> MMFGKKKNNGGSSTARYSAGNKYNTLSNNYALSAQQLLNASKIDDIDSMMGFERYVPPQYNGRFDAKDIDQIPGRVGWLTNMHATLVSQETLSSGSNGGGNSNDGERVTTNQGISGVDFYFLDEEGGSFKSTVVYDPYFFIACNDESRVNDVEELVKKYLESCLKSLQIIRKEDLTMDNHLLGLQKTLIKLSFVNSNQLFEARKLLRPILQDNANNNVQRNIYNVAANGSEKVDAKHLIEDIREYDVPYHVRVSIDKDIRVGKWYKVTQQGFIEDTRKIAFADPVVMAFDIETTKPPLKFPDSAVDQIMMISYMIDGEGFLITNREIISEDIEDFEYTPKPEYPGFFTIFNENDEVALLQRFFEHIRDVRPTVISTFNGDFFDWPFIHNRSKIHGLDMFDEIGFAPDAEGEYKSSYCSHMDCFRWVKRDSYLPQGSQGLKAVTQSKLGYNPIELDPELMTPYAFEKPQHLSEYSVSDAVATYYLYMKYVHPFIFSLCTIIPLNPDETLRKGTGTLCEMLLMVQAYQHNILLPNKHTDPIERFYDGHLLESETYVGGHVESLEAGVFRSDLKNEFKIDPSAIDELLQELPEALKFSVEVENKSSVDKVTNFEEIKNQITQKLLELKENNIRNELPLIYHVDVASMYPNIMTTNRLQPDSIKAERDCASCDFNRPGKTCARKLKWAWRGEFFPSKMDEYNMIKRALQNETFPNKNKFSKKKVLTFDELSYADQVIHIKKRLTEYSRKVYHRVKVSEIVEREAIVCQRENPFYVDTVKSFRDRRYEFKGLAKTWKGNLSKIDPSDKHARDEAKKMIVLYDSLQLAHKVILNSFYGYVMRKGSRWYSMEMAGITCLTGATIIQMARALVERVGRPLELDTDGIWCILPKSFPETYFFTLENGKKLYLSYPCSMLNYRVHQKFTNHQYQELKDPLNYIYETHSENTIFFEVDGPYKAMILPSSKEEGKGIKKRYAVFNEDGSLAELKGFELKRRGELQLIKNFQSDIFKVFLEGDTLEGCYSAVASVCNRWLDVLDSHGLMLEDEDLVSLICENRSMSKTLKEYEGQKSTSITTARRLGDFLGEDMVKDKGLQCKYIISSKPFNAPVTERAIPVAIFSADIPIKRSFLRRWTLDPSLEDLDIRTIIDWGYYRERLGSAIQKIITIPAALQGVSNPVPRVEHPDWLKRKIATKEDKFKQTSLTKFFSKTKNVPTMGKIKDIEDLFEPTVEEDNAKIKIARTTKKKAVSKRKRNQLTNEEDPLVLPSEIPSMDEDYVGWLNYQKIKWKIQARDRKRRDQLFGNTNSSRERSALGSMIRKQAESYANSTWEVLQYKDSGEPGVLEVFVTINGKVQNITFHIPKTIYMKF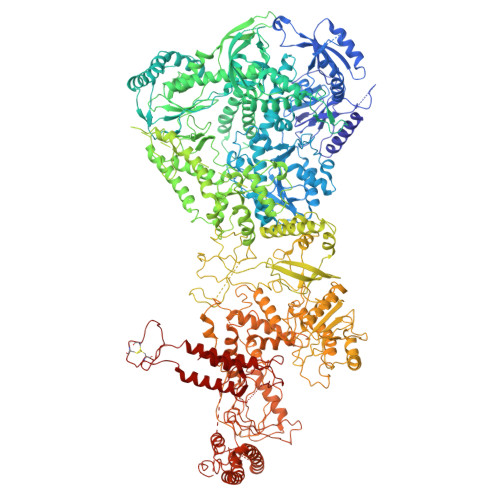KSQTMPLQKIKNCLIEKSSASLPNNPKTSNPAGGQLFKITLPESVFLEEKENCTSIFNDENVLGVFEGTITPHQRAIMDLGASVTFRSKAMGALGKGIQQGFEMKDLSMAENERYLSGFSMDIGYLLHFPTSIGYEFFSLFKSWGDTITILVLKPSNQAQEINASSLGQIYKQMFEKKKGKIETYSYLVDIKEDINFEFVYFTDISKLYRRLSQETTKLKEERGLQFLLLLQSPFITKLLGTIRLLNQMPIVKLSLNEVLLPQLNWQPTLLKKLVNHVLSSGSWISHLIKLSQYSNIPICNLRLDSMDYIIDVLYARKLKKENIVLWWNEKAPLPDHGGIQNDFDLNTSWIMNDSEFPKINNSGVYDNVVLDVGVDNLTVNTILTSALINDAEGSDLVNNNMGIDDKDAVINSPSEFVHDAFSNDALNVLRGMLKEWWDEALKENSTADLLVNSLASWVQNPNAKLFDGLLRYHVHNLTKKALLQLVNEFSALGSTIVYADRNQILIKTNKYSPENCYAYSQYMMKAVRTNPMFSYLDLNIKRYWDLLIWMDKFNFSGLACIEIEEKENQDYTAVSQWQLKKFLSPIYQPEFEDWMMIILDSMLKTKQSYLKLNSGTQRPTQIVNVKKQDKEDSVENSLNGFSHLFSKPLMKRVKKLFKNQQEFILDPQYEADYVIPVLPGSHLNVKNPLLELVKSLCHVMLLSKSTILEIRTLRKELLKIFELREFAKVAEFKDPSLSLVVPDFLCEYCFFISDIDFCKAAPESIFSCVRCHKAFNQVLLQEHLIQKLRSDIESYLIQDLRCSRCHKVKRDYMSAHCPCAGAWEGTLPRESIVQKLNVFKQVAKYYGFDILLSCIADLTI> NALKPAFGPPDKVAAQKFKESLMATEKHAKDTSNMWVKISVWVALPAIALTAVNTYFVEKEHAEHREHLKHVPDSEW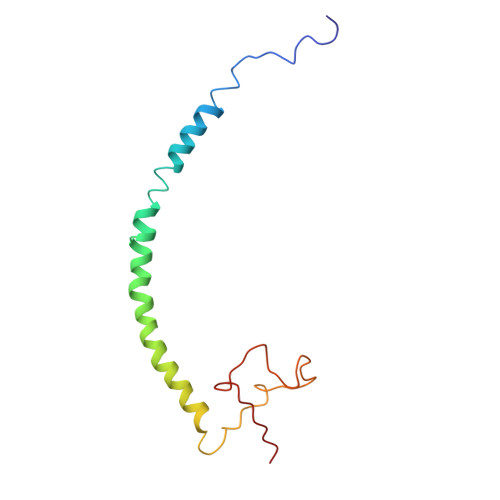PRDYEFMNIRSKPFFWGDGDKTLFWNPVVNRHIEHDD> KQRIDLRLTDDDKSMIEEAAAISNQSVSQFMLNSASQRAAEVIEQHRRVILNEESWTRVMDALSNPPSPGE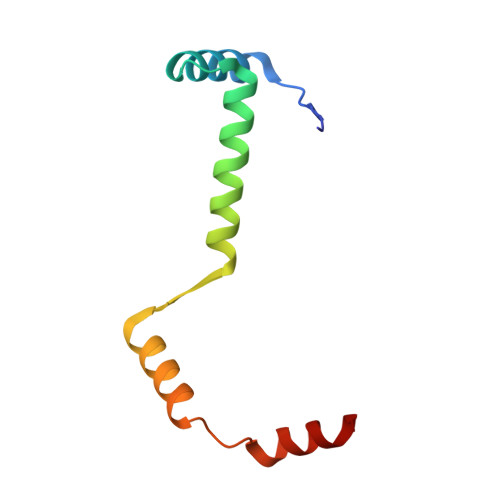KLKRAAKRLQ> MNIFRLTGDLSHLAAIIILLLKIWKSRSCAGISGKSQLLFALVFTTRYLDLFTSFISLYNTSMKLIYIACSYATV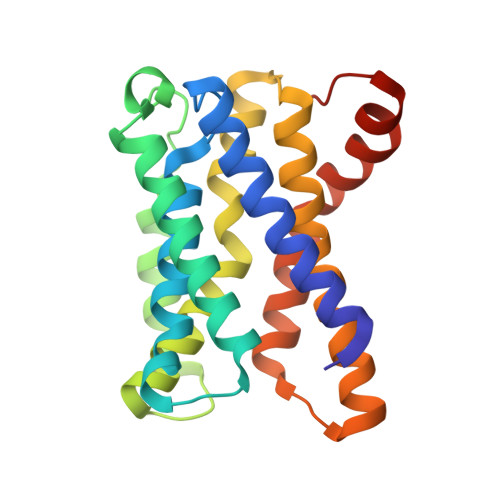YLIYMKFKATYDGNHDTFRVEFLIVPVGGLSFLVNHDFSPLEILWTFSIYLESVAILPQLFMISKTGEAETITTHYLFFLGLYRALYLVNWIWRYYFEGFFDLIAVVAGVVQTVLYCDFFYLYVTKVLKGKKLSLPA> PIETVPVKLKPGMDGPKVKQWPLTEEKIKALVEICTEMEKEGKISKIGPENPYNTPVFAIKKKDSTKWRKLVDFRELNKRTQDFWEVQLGIPHPAGIKKKKSVTVLDVGDAYFSVPLDEDFRKYTAFTIPSINNETPGIRYQYNVLPQGWKGSPAIFQSSMTKILEPFRKQNPDIVIYQYMDDLYVGSDLEIGQHRTKIEELRQHLLRWGLTTPDKKHQK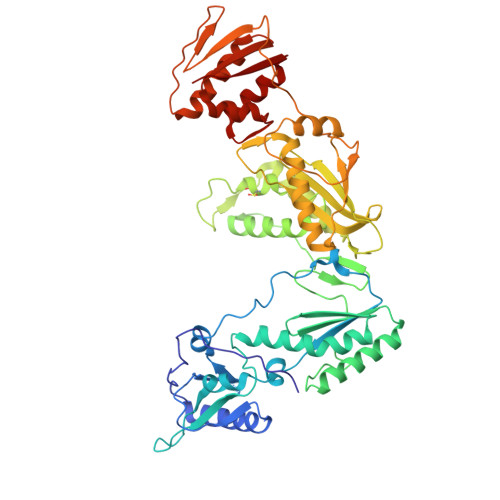EPPFLWMGYELHPDKWTVQPIVLPEKDSWTVNDIQKLVGKLNWASQIYPGIKVRQLCKLLRGTKALTEVIPLTEEAELELAENREILKEPVHGVYYDPSKDLIAEIQKQGQGQWTYQIYQEPFKNLKTGKYARMRGAHTNDVKQLTEAVQKITTESIVIWGKTPKFKLPIQKETWETWWTEYWQATWIPEWEFVNTPPLVKLWYQLEKEPIVGAETFYVDGAANRETKLGKAGYVTNRGRQKVVTLTDTTNQKTELQAIYLALQDSGLEVNIVTDSQYALGIIQAQPDQSESELVNQIIEQLIKKEKVYLAWVP>MSKKTIVSMAVIRRLPRYHRYLEELLKNDVKRISSRELSEKMGVTASQIRQDLNNFGGFGQQGYGYNVEELYNNLTKILGLDKTYNTIIIGAGNLGQAIANYTSFEKSGFNLKGIFDINPRLFGLKIRDV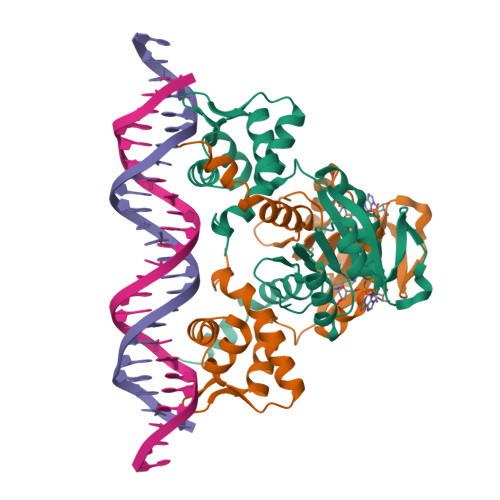EVMDVETVEDFIARNKIDIGILCIPKDNAQYTADRLVRAGIKAIWNFLPIDLKVPDDVILENVHLSDSLFTVSYRLNEEELFKKLKGETAKIDG[4x]> GIDPFTAKRTHRVINHPYYFPFNGRQAEDYLRSKERGEFVIRQ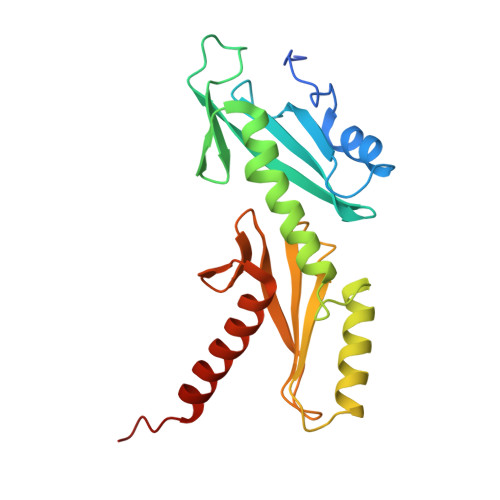SSRGDDHLVITWKLDKDLFQHIDIQELEKENPLALGKVLIVDNQKYNDLDQIIVEYLQNKVRLLNEMTSSEKFKSGTKKDVVKFIEDYSRVNPNKSVYYFSLNHDNPGWFYLMFKINANSKLYTWNVKLTNTGYFLVNYNYPSVIQLCNGFKTLLKSNSSKNRMNNYR>GSDEDTYYLQVRGRKNFEILMELKRSLELMELVPQPL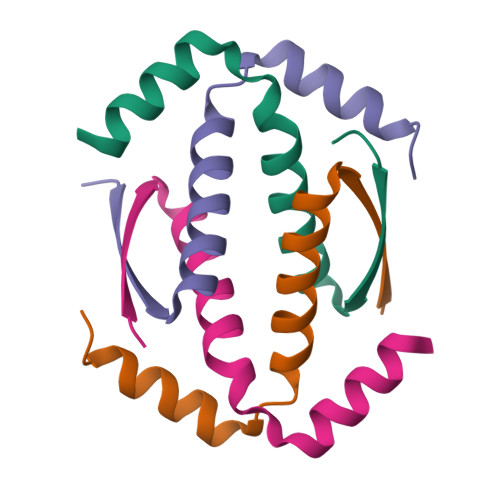VDSYEQQQQLLQR[8x]>[4x]MTSTGRFTLPSEENFAEKTKELAELWGADAIRNSDGTHLDEAVLALGKKIYNAYFPTRAHNEWITLHMDETPQVYLLTDRILAESDTVDIPLMESFFAEQLKPNRDADPHKYWEVVDRTTGEVVDSANWTLDADEDT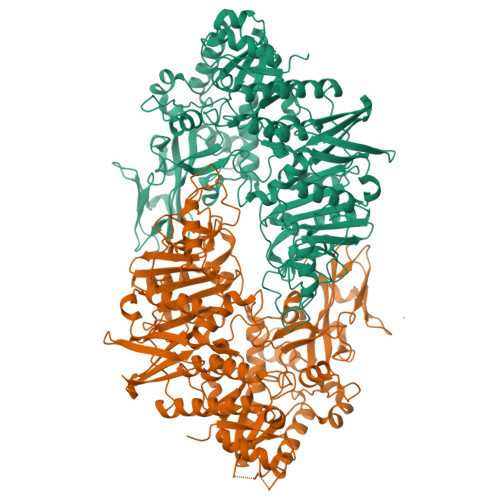VHVSGVAAWHEYTVSFLAYIIWDPVEMYNHLTNDWGDKEHEIPFDIYHPATRKFVFDTFEQWLKDSPQTDVVRFTTFFYQFTLLFDEKRREKVVDWFGCACTVSPRALDDFEAKYGYRLRPEDFVDGGAYNSAWRVPRKAQRDWIDFLSGFVRENVKQLADMSHAAGKEAMMFLGDQWIGTEPYKDGFDELGLDAVVGSIGDGTTTRMIADIPGVKYTEGRFLPYFFPDTFYEGNDPSIEGLDNWRKARRAILRSPISRMGYGGYLSLAAKFPKFVDTVTHIANEFRDIHDRTGGVAAEGELNVAILNSWGKMRSWMAFTVAHALPNKQTYSYYGILESLSGMRVNVRFISFDDVLAHGIDSDIDVIINGGPVDTAFTGGDVWTNPKLVETVRAWVRGGGAFVGVGEPSSAPRFQTGRFFQLADVIGVDEERYQTLSVDKYFPPVVPDHFITADVPVDPAAREAWEQAGYRIPLSGCGGGQSIKPLGGIDFGEPVLNTYPVNENVTLLRADGGQVQLATNDYGKGRGVYISGLPYSAANARLLERVLFYASHNEDKYAAWSSSNPECEVAHFPEQGLYCVINNTDQPQKTTVTLADGTTEDFDLPDSGIAWREALEHHHHHH> DKMDYDFKVKLSSERERVEDLFEYEGCKVGRGTYGHVYKAKRKDGKDDKDYALKQIEGTGISMSACREIALLRELKHPNVISLQKVFLSHADRKVWLLFDYAEHDLWHIIKFHRASKANKKPVQLPRGMVKSLLYQILDGIHYLHANWVLHRDLKPANILVMGEGPERGRVKIADMGFARLFNSPLKPLADLDPVVVTFWYRAPELLLGARHYTKAIDIWAIGCIFAELLTSEPIFHCRQEDIKTSNPYHHDQLDRIFNVMGFPADKDWEDIKKMPEHSTLMKDFRRNTYTNCSLIKYMEKHKVKPDSKAFHLLQKLLTMDPIKRITSEQAMQDPYFLEDPLPTSDVFAGCQIPYPKREFLTEE;> KAMAGNFWQSSHYLQWILDKQDLLKERQKDLKFLSEEEYWKLQIFFTNV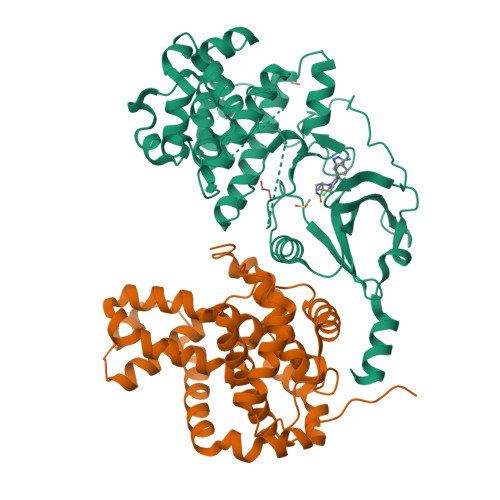IQALGEHLKLRQQVIATATVYFKRFYARYSLKSIDPVLMAPTCVFLASKVEEFGVVSNTRLIAAATSVLKTRFSYAFPKEFPYRMNHILECEFYLLELMDCCLIVYHPYRPLLQYVQDMGQEDMLLPLAWRIVNDTYRTDLCLLYPPFMIALACLHVACVVQQKDARQWFAELSVDMEKILEIIRVILKLYEQWKNFDERKEMATILSKMPKPKPPP> RTEDLPKAVVFLEPQWYRVLEKDSVTLKCQGAY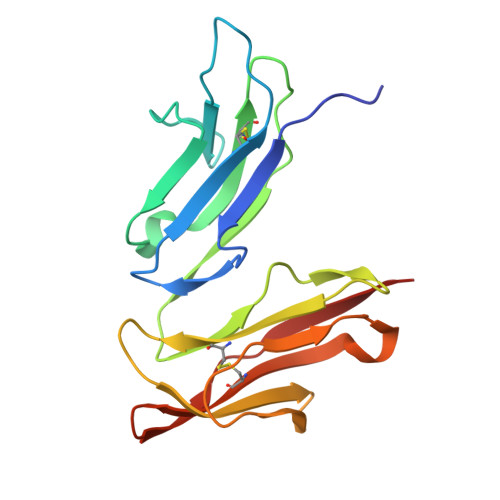SPEDNSTQWFHNESLISSQASSYFIDAATVDDSGEYRCQTNLSTLSDPVQLEVHIGWLLLQAPRWVFKEEDPIHLRCHSWKNTALHKVTYLQNGKGRKYFHHNSDFYIPKATLKDSGSYFCRGLVGSKNVSSETVNITITQG> GSHMSQLYASL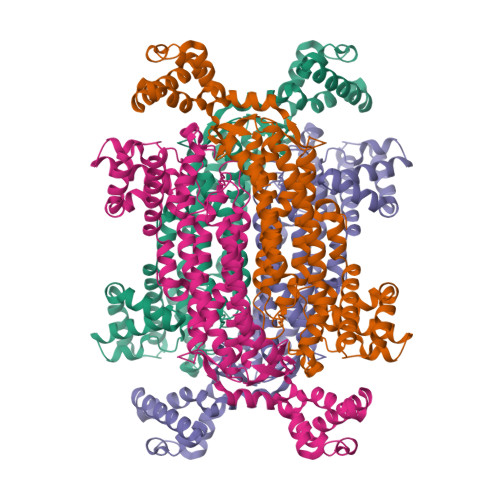FYQRDVTEIFSDRALVSYMVEAEVALAQAQAQVGVIPQSAATVIQRAAKTAIDKIDFDALATATGLAGNIAIPFVKQLTAIVKDADEDAARYVHWGATSQDILDTACILQCRDALAIVQNQVQQCYETALSQAQTYRHQVMMGRTWLQQALPITLGHKLARWASAFKRDLDRINAIKARVLVAQLGGAVGSLASLQDQGSIVVEAYAKQLKLGQTACTWHGERDRIVEIASVLGIITGNVGKMARDWSLMMQTEIAEVFEPTAKGRGGSSTMPHKRNPVAAASVLAAANRVPALMSSIYQSMVQEHERSLGAWHAEWLSLPEIFQLTAGALERTLDVLKGMEVNAENMHQNIECTHGLIMAEAVMMALAPHMGRLNAHHVVEAACKTAVAEQKHLKDIISQVDEVKQYFNPSQLDEIFKPESYLGNIQDQIDAVLQEAKGEAK1,1'-[ethane-1,2-diylbis(oxyethane-2,1-diyl)]bis(1H-pyrrole-2,5-dione) | C14 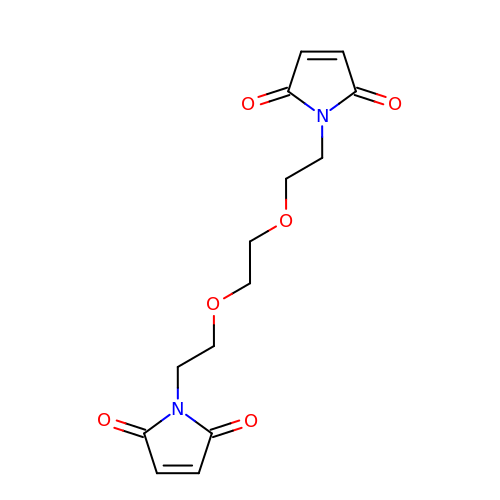H16 N2 O6 | FERLGYOHRKHQJP-UHFFFAOYSA-N>GSHMTNRLVLSGTVCRAPLRKVSPSGIPHCQFVLEHRSVQEAAGFHRQAWCQMPVIVSGHENQ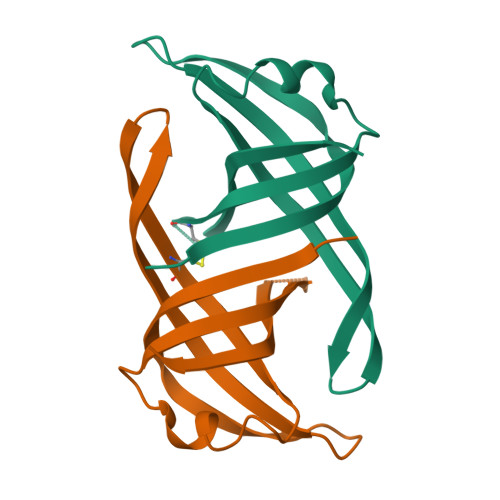AITHSITVGSRITVQGFISCHKAKNGLSKMVLHAEQIELIDSGD[2x]>[2x]ARVAINGFGRIGRLVYRII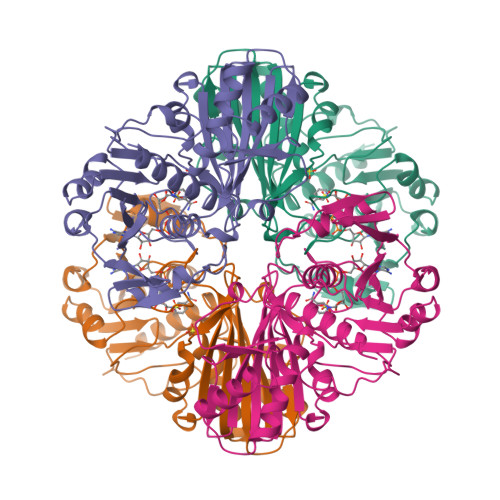YERKNPDIEVVAINDLTDTKTLAHLLKYDSVHKKFPGKVEYTENSLIVDGKEIKVFAEPDPSKLPWKDLGVDFVIESTGVFRNREKAELHLQAGAKKVIITAPAKGEDITVVIGCNEDQLKPEHTIISCASCTTNSIAPIVKVLHEKFGIVSGMLTTVHSYTNDQRVLDLPHKDLRRARAAAVNIIPTTTGAAKAVALVVPEVKGKLDGMAIRVPTPDGSITDLTVLVEKETTVEEVNAVMKEATEGRLKGIIGYNDEPIVSSDIIGTTFSGIFDATITNVIGGKLVKVASWYDNEYGYSNRVVDTLELLLKM> MPPAPPDQKPCHQLQPAPYRALSESILFGSVDEERWWHSTAPILSRLLISSNYDVDVQYKYLSLYRHLVLPALGPYPQRDPETGII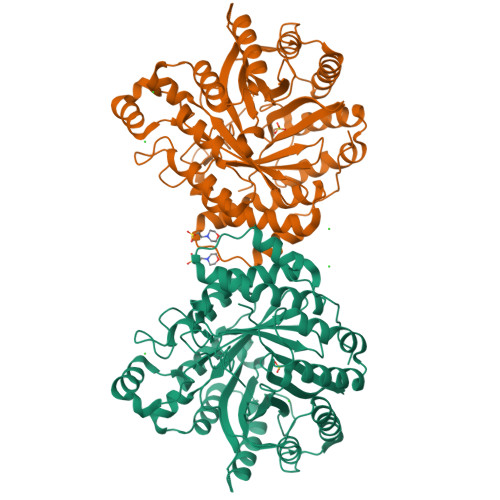ATQWRSGMVLTGLPIEFSNNVARALIRIGVDPVTADSGTAQDPFNTTRPKVYLETAARLLPGVDLTRFYEFETELVITKAEEAVLQANPDLFRSPWKSQILTAMDLQKSGTVLVKAYFYPQPKSAVTGRSTEDLLVNAIRKVDREGRFETQLANLQRYIERRRRGLHVPGVTADKPPATAADKAFDACSFFPHFLSTDLVEPGKSRVKFYASERHVNLQMVEDIWTFGGLRRDPDALRGLELLRHFWADIQMREGYYTMPRGFCELGKSSAGFEAPMMFHFHLDGSQSPFPDPQMYVCVFGMNSRKLVEGLTTFYRRVGWEEMASHYQANFLANYPDEDFEKAAHLCAYVSFAYKNGGAYVTLYNHSFNPVGDVSFPNGSRSHHHHHH> VIPDYFKQSFPEGYSWERSMTYEDGGICIATNDITMEGDSFINKIHFKGTNFPPNGP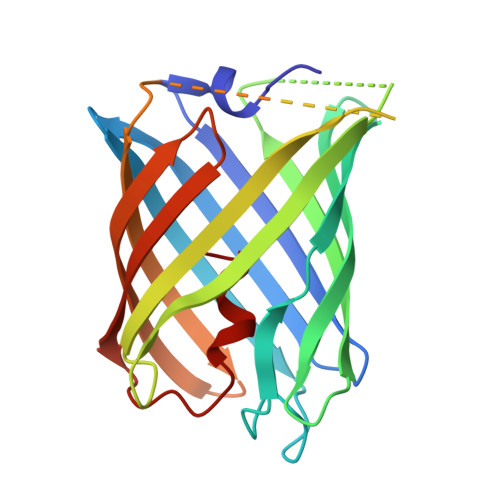VMQKRTVGWEASTEKMYERDGVLKGDVKMKLLLKGGGHYRCDYRTTYKVKQKPVKLPDYHFVDHRIEILSHDKDYNKVKLYEHAVARNSTDSMDELYKGGSGGMVSKGEETITSVIKPDMKNKLRMEGNVNGHAFVIEGEGSGKPFEGIQTIDLEVKEGAPLPFAYDILTTAFF> GLMAASTEGVISNKQVILKDYVTGFPKESDMQLTTATTKLKLPEGSKGVLVKNLYLSCDPYMRSRMTKREPGASYVDSFDAGSPIVGYGVAKVLESGDPKFKKGDLIWGMTGWEEYSVITSTESLFKIQHIDVPLSYYTGILGMPGMTAYAGFYEICNPKKGETVFVSAASGAVGQLVGQFAKLLGCYVVGSAGSKEKVDLLKNKFGFDNAFNYKEEPDLDAALKRYFPEGIDIYFENVGGVMLDAVLPNMRVHGRIAVCGLISQYNIAAAEGCRNLMYLIIKQVRMQGFLVFSYYHLYEKFLEMVLPAIKEGKLTYVEDVVEGLESAPAALIGLY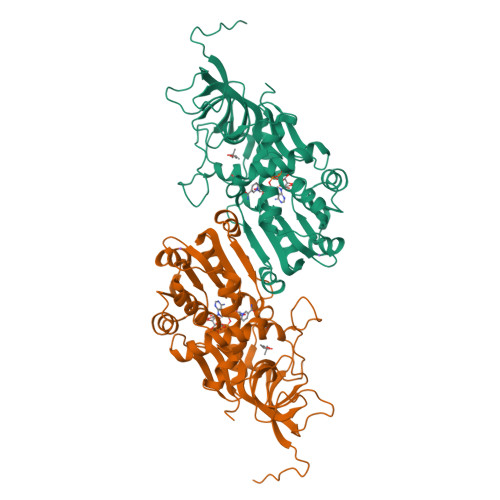AGRNVGKQVVVVSRE>MSVDPNQYYKIRSQAIHQLKVNGEDPYPHKFHVDISLTDFIQKYSHLQPGDHLTDITLKVAGRIHAKRASGGKLIFYDLRGEGVKLQVMANSRNYKSEEEFIHINNKLRRGDIIGVQGNPGKTKKGELSIIPYEITLLSPCLHMLPHLHFGLKDKETRYRQRYLDLILNDFVRQKFIIRSKIITYIRSFLDELGFLEIETPMMNIIPGGAVAKPFITYHNELDMNLYMRIATELYHKMLVVGGIDRVYEIGRVFRNEGIDLTHNPEFTSCEFYMAYADYHDLMEITE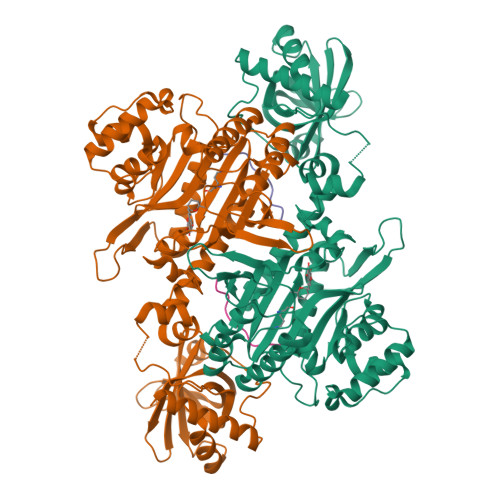KMVSGMVKHITGSYKVTYHPDGPEGQAYDVDFTPPFRRINMVEELEKALGMKLPETNLFETEETRKILDDICVAKAVECPPPRTTARLLDKLVGEFLEVTCINPTFICDHPQIMSPLAKWHRSKEGLTERFELFVMKKEICNAYTELNDPMRQRQLFEEQAKAKAAGDDEAMFIDENFCTALEYGLPPTAGWGMGIDRVAMFLTDSNNIKEVLLFPAMKPEDKKEN[4x];>MPMYQVKPYHGGGAPLRVELPTCMYRLPNVHGRSYGHHHHHH[4x]(1R,3S,5Z)-5-[(2E)-2-[(1R,3aS,7aR)-1-[(2R,6S)-6-(1-adamantyl)-6-oxidanyl-hex-4-yn-2-yl]-7a-methyl-2,3,3a,5,6,7-hexahydro-1H-inden-4-ylidene]ethylidene]-4-methylidene-cyclohexane-1,3-diol 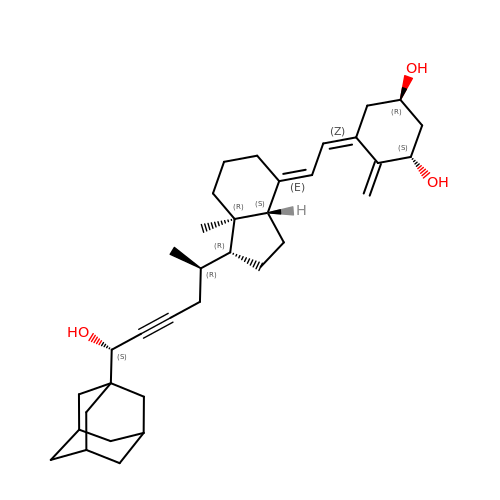| C35 H50 O3 | RKVGVUCXMUXZTG-LLLPRGGASA-N>MAHHHHHHMKPILIGLIMGSQSDWQTLIHAAHTLDALNIGYEAEIVSAHRTPDKLFRYAEQAEARGLEVIIAGAGGAAHLPGMVAAKTSLPVLGVPVMSQTLNGVDSLLSIVQMPAGIPVGTLSIGKAGAINSALFAAAILANKYPDIRAALKHYREQQTQKVLDNPNPK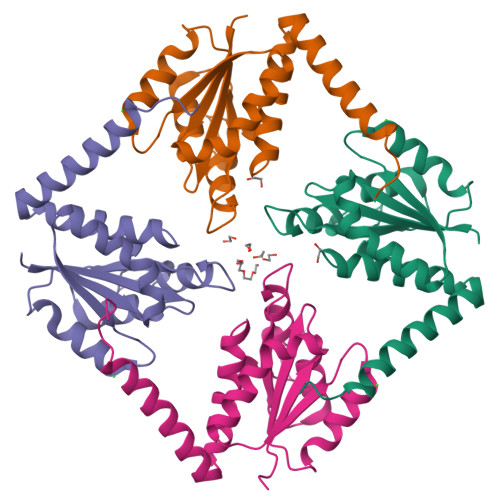EEKS[4x]>VIGDLKCNTSSINDVDTGVPSISSEVVDVTNGLGTFYVLDRVYLNTTLLLNGYYPISGATFRNMALKGTRLLSTLWFKSPFLSPFNDGIFAKVKNSRFSKDGVIYSEFPAITIGSTFVNSSHSIVVKPHTSFINGNLQGLLQISVCQYTMCEYPHTICHPNLGNQRIELWHYDTDVVSCLYKRNFTYDVNADYLYFHFYQEGGTFYAYFTDTGFVTKFLFKLYLGTVLSHYYVMPLTCDSALSLEYWVTPLTTRQFLLA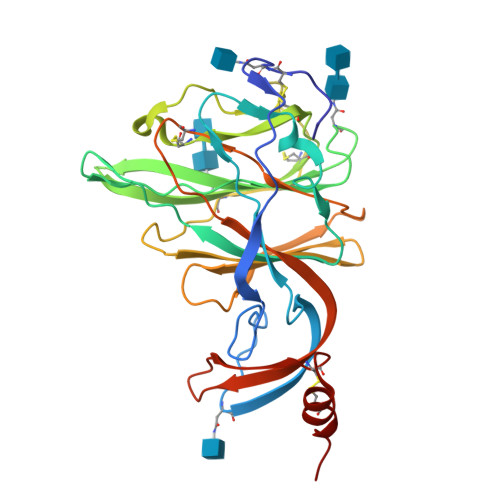FDQDGVLYHAVDCASDFMSEIMCKTSSDP[2x]> MEAICSSLEPLFPCREAAIETLGELIGDSSETYPSAIYLFGHSGTGKTALTRAFLKECGKRQNVRTAHLNAIECYTTKIMLEILLDSLAPDQGDALKVDNMLDFVEQLRRQAATRVEDQGFLIAVDNAERLRDMDANVLPVLLRLQELTNLNLCVILLSQLPFEKFYNKTGLSEIVCLHLAQYNKAETQRILGSDFQQVRNQLLEQFAQDKKRLEICQEAVTEDFYNNYLNLFLSVFYKACRDVPELQLTARKCLSTYLEPVLDGTVDATDISRLWRHIAGPLRSALTQIYMRIEKPAEEVEDFTAIEDQSVRKLAQSLELPYYAKFLLIAAFLASHNAAKQDKRLFVKHHGKQRKRMQTVNARAKTTEKM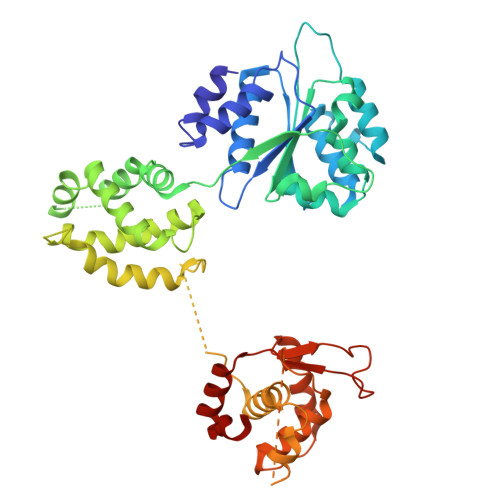STTLGPKSFSIDRLLAIFYAILEEKVGLTCNLLSQISTLVHLNLLSFVSGEQNIMEGSARLQCTIGLEFVLQIGKVVGFNVRQYLCDFM> MSVEGLGKDFCGAIIPDNFFPIEKLRNYTQMGLIRDFAKGSAVIMPGEEITSMIFLVEGKIKLDIIFEDGSEKLLYYAGGNSLIGKLYPTGNNIYATAMEPTRTCWFSEKSLRTVFRTDEDMIFEIFKNYLTKVAYYARQVAEMNTYNPTIRILRLFYELCSSQGKRVGDTYEITMPLSQKSIGEITGVHHVTVSRVLASLKRENILDKKKNKIIVYNLGELKHLSEQTSYYSDPNSSSVDKLAAALDHH

The transcriptional regulator CprK from Desulfitobacterium spp. induces expression of halorespiratory genes upon binding of o-chlorophenol ligands and is reversibly inactivated by oxygen through disulphide bond formation. The CprK associated with the o-chlorophenolacetic acid (OCPA) reductive dehalogenase (CprAB) from D. dehalogenans and the closely related D. hafniense has been shown to bind OCPA with μM affinity leading to sequence-specific DNA-binding, and ultimately transcriptional activation of the associated cpr gene cluster (Pop et al., 2004; 2006; Gabor et al., 2006; Joyce et al., 2006; Mazon et al., 2007). Members of this family are homodimeric and contain an N-terminal sensor domain linked via a long α-helix (involved in formation of the dimer interface) to the C-terminal helix–turn–helix (HTH) DNA-binding domain. We here present crystal structures of the oxidized ligand-free (3.2 Å) and reduced ligand-free (2.0 Å), OCPA-bound (1.8 Å) and DNA-bound (1.8 Å) D. hafniense CprK in addition to an intermediate OCPA-bound structure obtained by soaking ligand-free crystals (2.0 Å).

The 1.8 Å crystal structure of CprKC200S in complex with a palindromic 30 bp dsDNA fragment containing the consensus (de)halobox sequence (as determined by in vivo promoter analysis; DNA sequence CCGGCATGTTAATGCGCATTAACATGCCGG, (de)halobox consensus sequence in bold) could be obtained by cocrystallization. The asymmetric unit contains a single CprK monomer bound to the corresponding half of the (de)halobox DNA, with the CprK dimer and complete (de)halobox DNA related by crystal symmetry. No significant changes could be observed for the majority of the CprK structure when comparing the DNA-bound form with the CprKC200S:OCPA complex structures. However, in contrast to the latter, the CprK C-terminus region has become structured and is now in close contact with the DNA (de)halobox. As observed with CRP–DNA complexes, the DNA helix displays significant curvature (to approximately 80°) with the individual hinge points occurring at consensus sequence positions. A large proportion of the polar contacts established at the protein–DNA interface are made between the phosphate backbone and the protein, a subset that includes contacts made with residues from the C-terminal region (residues 227–232) that is disordered in the DNA-free structures. The C-terminal Tyr-230 together with Thr-193 establishes a hydrogen bond network with A18 and T19 that includes a structural water molecule. It is likely that this particular interaction is responsible for the requirement of a purine and a pyrimidine at positions 18 and 19 respectively. In contrast, the hydrophobic contacts established between Val-192 of the recognition helix and T20 clearly leads to the strict requirement for a pyrimidine at this position.4-[(2-azanyl-6-oxidanylidene-1,9-dihydropurin-8-yl)sulfanylmethyl]-3-fluoranyl-benzenecarbonitrile 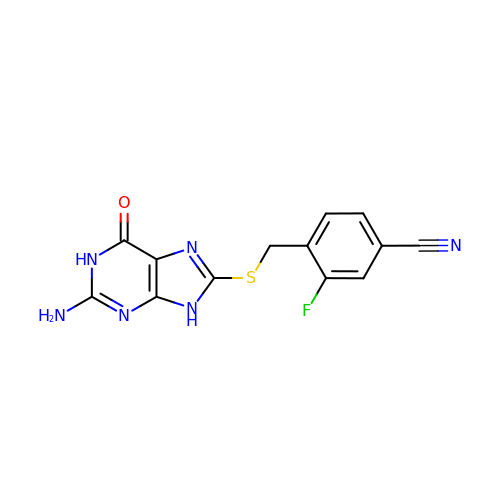| C13 H9 F N6 O S | GEUVDHJEINQZML-UHFFFAOYSA-N ATAs transfer an amino group of a chiral amine compound to a ketone compound using the cofactor pyridoxal 5’-phosphate (PLP) with a high turnover rate, stable catalytic activity, broad substrate specificity and excellent stereoselectivity, which is achieved by a proposed large-binding pocket (L pocket) and small-binding pocket (S pocket) in the substrate-binding site8910111213141516. Each protomer (subunit) of the dimeric enzymes shows a structural architecture typical of the fold-type IV class of PLP-dependent enzymes, which are made up of two domains. The substrate-binding site is surrounded by the cavity among the two domains, the cofactor PLP, and the loop consisting of the residues 129–145 of the other protomer. The substrate-binding site can be divided into two parts as described initially, the L pocket and the S pocket, which is consistent with the previously proposed mechanism for the substrate specificity of ATAs in which the smaller and larger atomic groups of substrates are recognized by the S and L pockets, respectively.

An improved R-ATA, designated as ATA-117-Rd11 was derived from ATA-117, a homolog of Ab-R-ATA, by the substrate walking approach for use in the synthesis of sitagliptin, on an industrial scale, whereas both Ab-R-ATA and ATA-117 could not produce such a large compounds. The molecular engineering of ATA-117-Rd11 involved 27 mutations that made this ATA conquer the severe reaction problems in the realistic industrial production, such as a high concentration of organic solvent, a high temperature for enhancing the solubility of prositagliptin ketone, and a high concentration of amine donor isopropylamine for prompting the product accumulation. In the final biocatalyst ATA-117-Rd11, Val69, Phe122, and Ala284 (in the S pocket of Ab-R-ATA) were mutated to Thr, Met, and Gly, respectively. Comparison of the active site pockets of the Ab-R-ATA and ATA-117-Rd11 shows that the volume of S pocket is enlarged by the three mutations. Similarly, His62 (in the L pocket of Ab-R-ATA) was mutated to Thr to increase the volume of the active site around it by reducing the volume of the amino acid side chain. The loops 129–145 of the G136F mutant and ATA-117-Rd11 showed significantly different conformation from that of the wild-type, depending on the amino acid residue at the position 136. Gly136 was located near Val152 in the wild-type, whereas Phe136 was distant from Val152 in the G136F mutant and ATA-117-Rd11, accompanied by the long-range alteration of the loop’s backbone conformation. The residue 136 was moved into the L pocket by the alteration of the loop, leading to a probable hydrophobic interaction between Phe136 and the cyclic group of pro-sitagliptin ketone. Simultaneously, Arg138 was moved away from the substrate-binding site by the alteration of the loop, resulting in an enlargement of the cavity to accommodate large substrates.

>MAFSADTPEIVYTHDTGLDYITYSDYELDPANPLAGGAAWIEGAFVPPSEARISIFDQGFYTSDATYTTFHVWNGNAFRLGDHIERLFSNAESIRLIPPLTQDEVKEIALELVAKTELREAMVTVTITRGYSSTPFERDITKHRPQVYMSACPYQWIVPFDRIRDGVHLMVAQSVRRTPRSSIDPQVKNFQWGDLIRAIQETHDRGFELPLLLDCDNLLAEGPGFNVVVIKDGVVRSPGRAALPGITRKTVLEIAESLGHEAILADITPAELYDADEVLGCSTGGGVWPFVSVDGNSISDGVPGPVTQSIIRRYWELNVEPSSLLTPVQY[12x]>[4x]MGSSHHHHHHSQ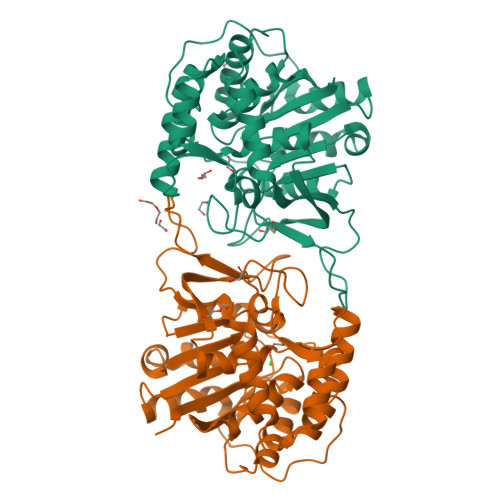DPNSSSMGQDGQQIRRDKLIIDTDPGIDDSMTILMAFRAPSVEIIGLTTIFGNVDTKGATRNALLLCERAGCPEVPVAEGSHEPLKGGKPRVADFVHGSDGIGNLFLPAPSAKKVEESAADFLINKVSEFPGEVSVLALGPLTNVALAIKRDPSFASKVKKIVVLGGAFFAAGNVNPAAEANIHGDPEAADIVFTSGADIVVVGINITTQVCLTDEDLLELRNSKGKHAAFLYEMCKFYRDWHAKSDGFHGIFLHDPVSFTAVLHPEYFTFKKGVVRVETQGICTGHTLMDQGLKKWNSENPWSGYKPISVAWTVDVPKVISFIKKLLMAP>[4x]MGAVFKLMKSDFYEREDFMGEVEDMITLKDIF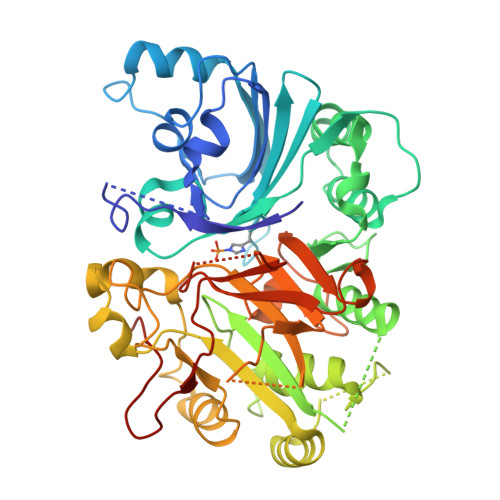GTETLKRSILFSFQYELDFLLRQFHQNVENITIVGQKGTIMPIEARAMDATLAVILKKVKLIEITMPPFASHHTKLIINFYDNGECKIFLPSNNFTSMETNLPQQVCWCSPLLKIGKEGLPVPFKRSLIEYLNSYHLKDIDELITKSVEEVNFAPLSELEFVYSTPSKFQSSGLLSFYNKLEKLSAGTSASDTAKHYLCQTSSIGTSLSRARDENLWTHLMIPLFTGIMSPPAKDTAGRKKAEILPTNSLINEYSQRKIKPYIIFPTEQEFVTSPLKWSSSGWFHFQYLQKKSYYEMLRNKFKVFYKQDPAMVTRRRGTTPARSKFYMHCATNSAGPCDASQVFKELEWCLYTSANLSQTAWGTVSRKPRNYEAGVLYHSRRLANTRKVTCRTFTRDRRGCAGNPTHVAVPFTLPVIPYDLAEDECFCLALHHHHHHH1-[6,7-dichloro-9-(1H-pyrazol-4-yl)-1,3,4,5-tetrahydro-2H-pyrido[4,3-b]indol-2-yl]-2-hydroxyethan-1-one 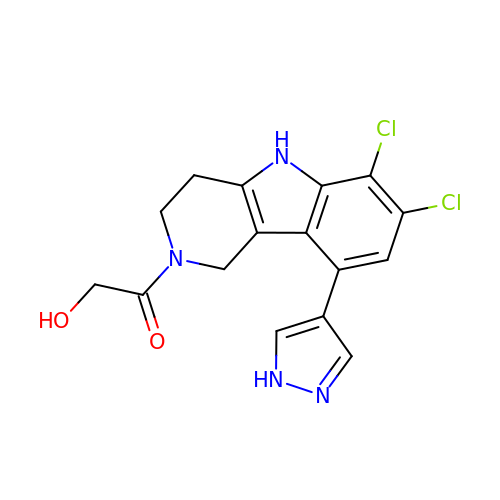| C16 H14 Cl2 N4 O2 | UUDFSTGSYHGEEV-UHFFFAOYSA-N> CAGCAGCCTGTACGGACATCA;> CCGTA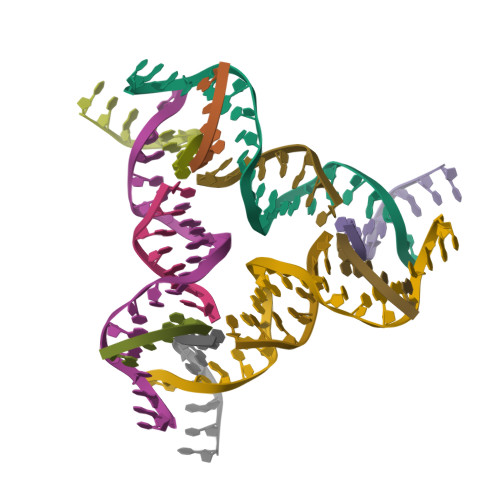CA;> GGCTG;> TCGTGATGT(2R)-4-[4-(3-methylphenyl)-1H-1,2,3-triazol-1-yl]-1-(2,4,5-trifluorophenyl)butan-2-amine 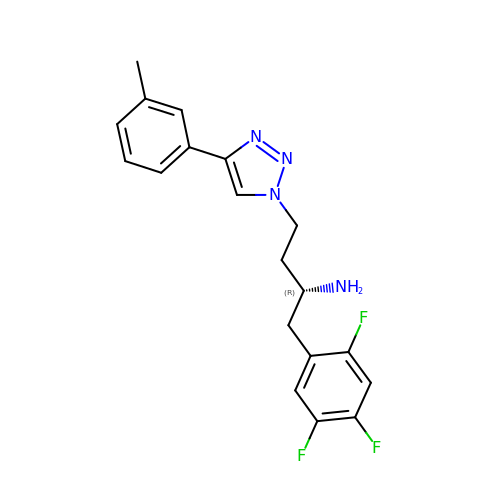| C19 H19 F3 N4 | BNUZDHPPDRXKCH-HNNXBMFYSA-N> MKKKGSVVIVGRINLSGDTAYAQQTRGEEGCQETSQTGRDKNQVEGEVQIVSTATQTFLATSINGVLWTVYHGAG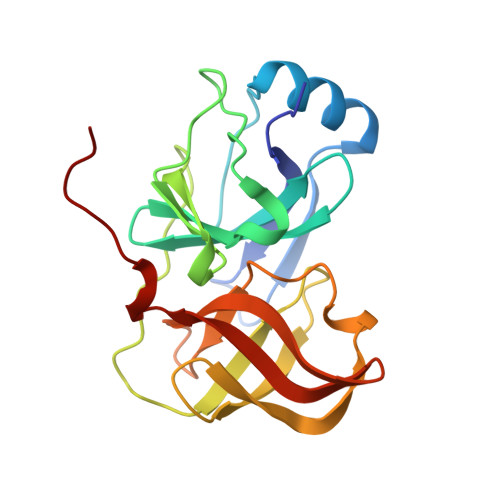TRTIASPKGPVTQMYTNVDKDLVGWQAPQGSRSLTPCTCGSSDLYLVTRHADVIPVRRRGDSRGSLLSPRPISYLKGSAGGPLLCPAGHAVGIFRAAVSTRGVAKAVDFIPVESLETTMRSP> MADRLTQLQDAVNSLADQFCNAIGVLQQCGPPASFNNIQTAINKDQPANPTEEYAQLFAALIARTAKDIDVLIDSLPSEESTAALQAASLYKLEEENHEAATCLEDVVYRGDMLLEKIQSALADIA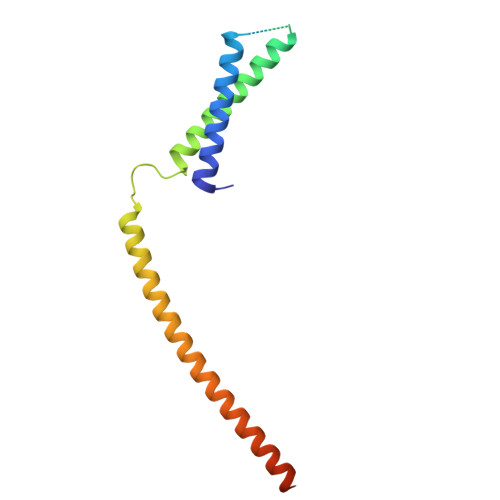QSQLKTRSGTHSQSLPDS>GMVVNESMYQLGSVRSAIRELFEYGKKRAAIVGKENVYDFSIGNPSIPAPQIVNDTIKELVTDYDSVALHGYTSAQGDVETRAAIAEFLNNTHGTHFNADNLYMTMGAAASLSICFRALTSDAYDEFITIAPYFPEYKVFVNAAGARLVEVPADTEHFQIDFDALEERINAHTRGVIINSPNNPSGTVYSEETIKKLSDLLEKKSKEIGRPIFIIADEPYREIVYDGIKVPFVTKYYDNTLVCYSYSKSLSLPGERIGYVLVPDEVYDKAELYAAVCGAGRALGYVCAPSLFQKMIVKCQGATGDINAYKENRD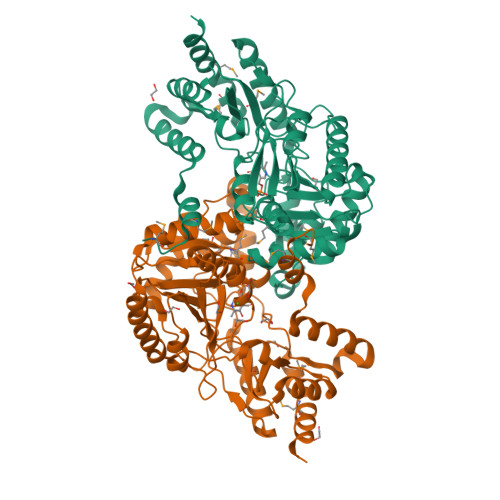LLYEGLTRIGYHCFKPDGAFYMFVKALEDDSNAFCEKAKEEDVLIVAADGFGCPGWVRISYCVDREMIKHSMPAFEKIYKKYNK[4x]>GG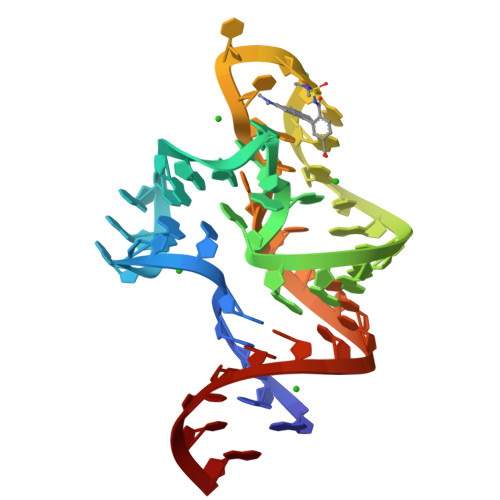ACUCGGAAACGUGAAGGAGAGGCGCAAGGUUAACCGCCUCAGUCCA[2x]> IVGGRKARPRQFPFLASIQNQGRHFCGGALIHARFVMTAASCFQSQNPGVSTVVLGAYDLRRR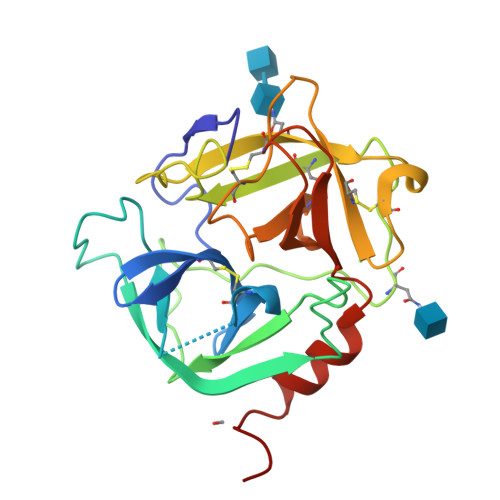ERQSRQTFSISSMSENGYDPQQNLNDLMLLQLDREANLTSSVTILPLPLQNATVEAGTRCQVAGWGSQRSGGRLSRFPRFVNVTVTPEDQCRPNNVCTGVLTRRGGICNGDQGTPLVCEGLAHGVASFSLGPCGRGPDFFTRVALFRDWIDGVLNNPGPGPA>[4x]MNSNLRGVMAALLTPFDQQQALDKASLRRLVQFNIQQGIDGLYVGGSTGEAFVQSLSEREQVLEIVAEEGKGKIKLIAHVGCVTTAESQQLAASAKRYGFDAVSAVTPFYYPFSFEEHCDHYRAIIDSADGLPMVVYNIPALSGVKLTLDQINTLVTLPGVGALKQTSGDLYQMEQIRREHPDLVLYNGYDEIFASGLLAGADGGIGSTYNIMGWRYQGIVKALKEG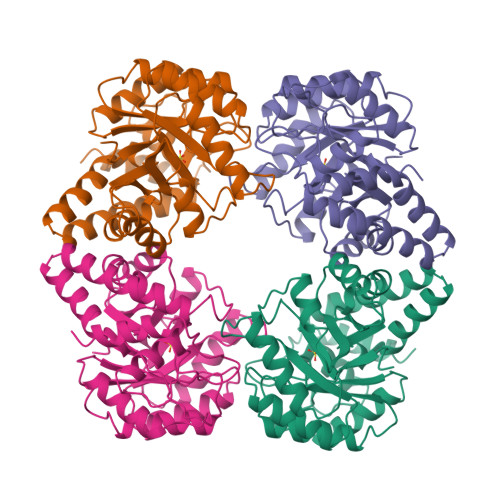DIQTAQKLQTECNKVIDLLIKTGVFRGLKTVLHYMDVVSVPLCRKPFGPVDEKYQPELKALAQQLMQERG> QTIGPGTGYSNGYYYSYWNDGHAGVTYTNGGGGSFTVNWSNSGNFVAGKGWQPGTKNKVINFSGSYNPNGNSYLSIYGWSRNPLIEYYIVENFGTYNPSTGATKLGEVTSDGSVYDIYRTQRVNQPSIIGTATFYQYWSVRRNHRSSGSVNTANHFNAWASHGLTLGT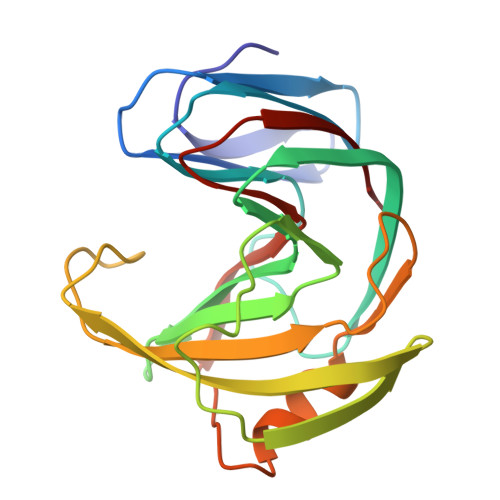MDYQIVAVEGYFSSGSASITVS> GPLGSTRAKTQEEIKREEEQAIDEVLKIEFLELALGYQLISLADMKQGGDLLERIRGIRKKIASDYGFLMPQIRIRDNLQLPPTHYEIKLKGIVIGEGMVMPDKFLAMNTGFVNREIEGIPTKEPAFGMDALWIDAKNKEEAIIQGYTIIDPSTVIATHTSELVKKYAEDFITKDEVKSLLERLAKDYPTIVEESKKIPTGAIRSVLQALLHEKIPIKDMLTILETITDIAPLVQNDVNILTEQVRARLSRVITNAFKSEDGRLKFLTFSTDSEQFLLNKLRENGTSKSLLLNVGELQKLIEGVSEEAMKVLQKGIAPVILIVEPNLRKALSNQMEQ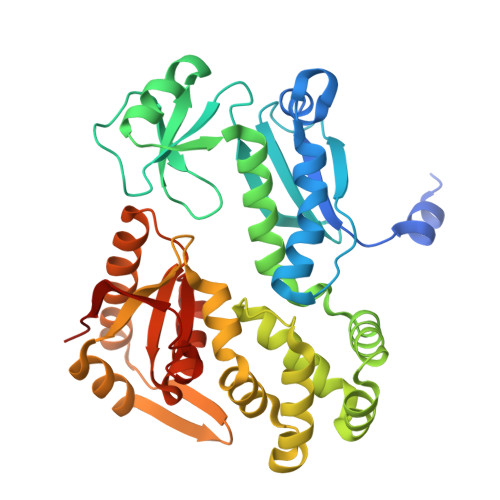ARIDVVVLSHAELDPNSNFEALGTIHIN> RTEDLPKAVVFLEPQWYSVLEKDSVTLKCQGAYSPEDNSTQWFHNESLISSQASSYFIDAATVNDSGEYRCQTNLSTLSDPVQLEVHIGWLLLQAPRWVFKEEDPIHLRCHSWKNTALHKVTYLQNGKDRKYFHHNSDFHIPKATLKDSGSYFCRGLVGS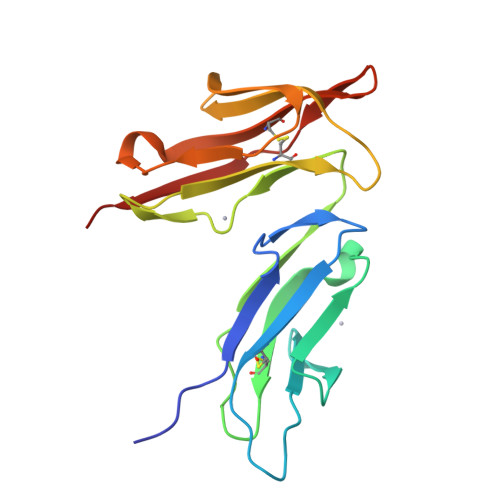KNVSSETVNITITQA>[4x]MATANGAVENGQPDRKPPALPRPIRNLEVKFTKIFINNEWHESKSGKKFATCNPSTREQICEVEEGDKPDVDKAVEAAQVAFQRGSPWRRLDALSRGRLLHQLADLVERDRATLAALETMDTGKPFLHAFFIDLEGCIRTLRYFAGWADKIQGKTIPTDDNVVCFTRHEPIGVCGAITPWNFPLLMLVWKLAPALCCGNTMVLKPAEQTPLTALYLGSLIKEAGFPPGVVNIVPGFGPTVGAAISSHPQINKIAFTGSTEVGKLVKEAASRSNLKRVTLELGGKNPCIVCADADLDLAVECAHQGVFFNQGQCCTAASRVFVEEQVYSEFVRRSVEYAKKRPVG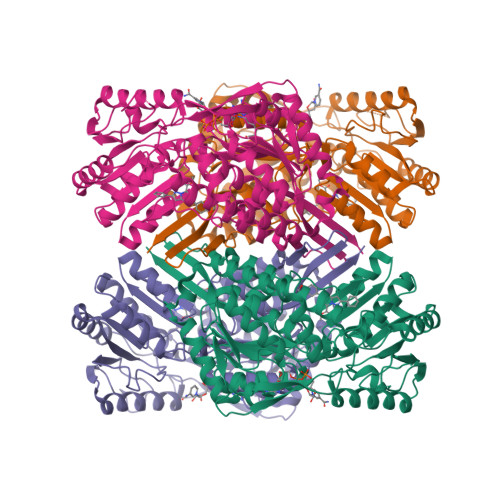DPFDVKTEQGPQIDQKQFDKILELIESGKKEGAKLECGGSAMEDKGLFIKPTVFSEVTDNMRIAKEEIFGPVQPILKFKSIEEVIKRANSTDYGLTAAVFTKNLDKALKLASALESGTVWINCYNALYAQAPFGGFKMSGNGRELGEYALAEYTEVKTVTIKLGDKNP> SMPRENIKGFSDAEIRRFIKSYKKFGGPLERLDAIARDAELVDKSETDLRRLGELVHNGCIKALKDSSSGTERTGGRLGKVKGPTFRISGVQVNAKLVISHEEELIPLHKSIPSDPEERKQYTIPCHTKAAHFDIDWGKEDDSNLLIGIYEYGYGSWEMIKMDPDLSL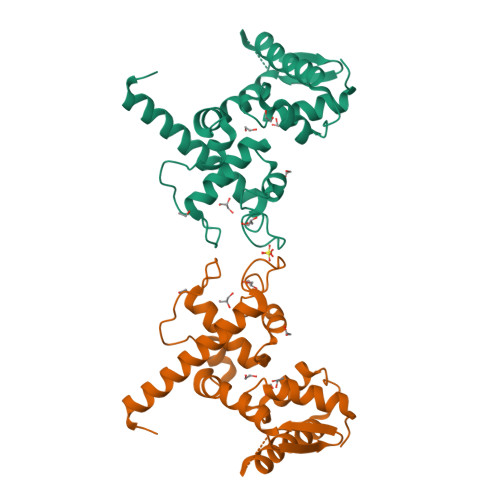THKILPDDPDKKPQAKQLQTRADYLIKLLSRDLAKKEALSGAG>MVNVAVNGYGTIGKRVADAIIKQPDMKLVGVAKTSPNYEAFIAHRRGIRIYVPQQSIKKFEESGIPVAGTVEDLIKTSDIVV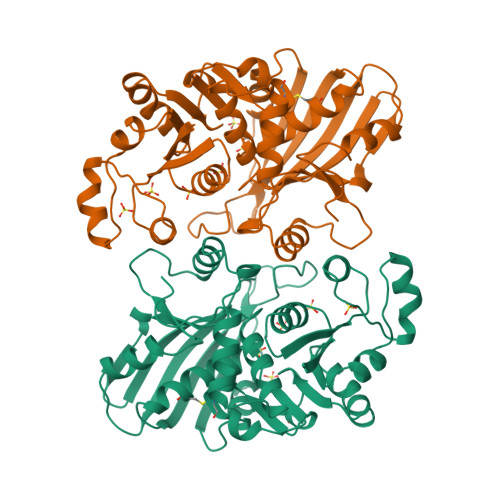DTTPNGVGAQYKPIYLQLQRNAIFQGGEKAEVADISFSALCNYNEALGKKYIRVVSCNTTALLRTICTVNKVSKVEKVRATIVRRAADQKEVKKGPINSLVPDPATVPSHHAKDVNSVIRNLDIATMAVIAPTTLMHMHFINITLKDKVEKKDILSVLENTPRIVLISSKYDAEATAELVEVARDLKRDRNDIPEVMIFSDSIYVKDDEVMLMYAVHQESIVVPENIDAIRASMKLMSAEDSMRITNESLGILKGYLI[2x]> ASTSCNVVLTDSQGSFTSPCYPNDYPPSQSCNWTIQAPAGFIVQITFLDFELEEAQGCIYDRVVVKTGTSDAKFCGLTANGLTLNSTGNVMEVFFNSDFSVQKKGFHISYKQVAVTLRNQKVTMPKSSKTILRVSNSISIPVLTAFTVCFEIARTAQKATETIFTLSDAAGTSILAFEKTSNGMELFIGASYCSVDNFLTSSDITATMKPLCLTWTKSSGLIGVYFEGHYFSSICSASQIYTLQSGGLLQIAGKGSSSVSVDDQNLDGFIYNFRLWDHAMLSSELSALTCDTVGNVVDWDHSYWTIPGSSTQTDSTLSCSTAITTLSPGTAGCASGLGCPEDIFYRSTLVVTDEQTPDRDATAIISQWLNQTFQNWMYRVYVDGISLQLITVLSRITTTRQIYLALLVYKNTTDVNLAEVEIESMLRSAPAIGNGLTLDSVTVNLMENCQADEFPVHYRWPESRPTVTQYVPCFPYKDRNASRTCMINRDNYTSFWALPDRGNCTNITSITVSQENAMDVAVQLADISNNGLSKEELTQVVTKVMELVNIAKINATLASTVVTIISNVMVSSEDAQKDASETALKAVDELVQKIEFDGPSLTISSKNLVVGVSALDTTNFNGSTLSAFIATNTTDPQIDFDSEAHNALAVVTLPPTLLQNLSLSQIEKVSRINFMFFGRTGLFQDHQNNGLTLNSYVVASSVGNFTIKNLQDPVRIEIAHLEYQKDPNPQCVFWDFNLQNYSGGWNSDGCKVGSDSNSNRTVCLCNHLTHFGILMDVSRAHHHHHHHH;> THFGILMDVSRA

Gpr126/Adgrg6 is one of the better studied aGPCRs and is essential for Schwann cell (SC) myelination and other functions. Gpr126 has a large ECR consisting of 839 aa. In this study, we determine the high-resolution crystal structure of the full-length ECR of zebrafish Gpr126, which reveals five domains, including a newly identified Sperm protein, Enterokinase and Agrin (SEA) domain, in which furin-mediated cleavage would occur in the human and mouse homologs. Intriguingly, the ECR is in an unexpected closed conformation that is reminiscent of the inactive closed conformation of the ECRs from EGFR and integrin families.

To determine the structure of the ECR of Gpr126, the full-length ECR (−ss) from zebrafish Gpr126 (T39-S837) was expressed and purified from insect cells using the baculovirus expression system. Zebrafish Gpr126 has high sequence identity (47%) to its human homolog but its ECR has a fewer number of N-linked glycosylation sites (15 predicted in zebrafish, 26 in human) and no furin-cleavage site, and thus yields a more homogeneous sample. Crystals of both native and selenomethionine (SeMet)-labeled zebrafish Gpr126 ECR (−ss) were obtained and diffracted to 2.4 Å, and the structure was determined by SeMet single-wavelength anomalous diffraction (SAD) phasing. The structure, with overall dimensions of 110 × 80 × 35 Å, revealed the presence of five domains, of which only four were identified previously. The 150 aa unknown region after the PTX domain was revealed to be a 22 aa linker that is partially disordered, the 23 aa alternatively spliced region (not present in crystal structure construct), and a structured domain which spans 105 aa and was identified as a SEA domain through the Dali server. Finally, the SEA domain is followed by the HormR and GAIN domains, the latter of which is autoproteolyzed as expected. Unexpectedly, the structure revealed a compact, closed conformation where the most N-terminal CUB domain interacts with the more C-terminal HormR and GAIN domains. As the closed conformation of Gpr126 (−ss) ECR was shown to exist both in solution and in the crystal lattice, we next wanted to explore the interactions that contribute to this protein architecture. Close examination of the crystal structure revealed two interaction sites that mediate the closed conformation, the first of which is a direct interaction between domains that are at opposite ends of the ECR and the second is an indirect interaction formed between two domains through a loop that holds them together. Residues in the HormR domain (H516, F533, P534, Y535) interact with each other through pi-pi stacking (sandwich), promoting interaction with F135 on the CUB domain through additional (T-shaped) pi-pi stacking to stabilize the CUB-HormR interaction.7-(2,4-DIAMINO-6-ETHYLPYRIMIDIN-5-YL)-1-(3-METHOXYPROPYL)QUINOLINIUM 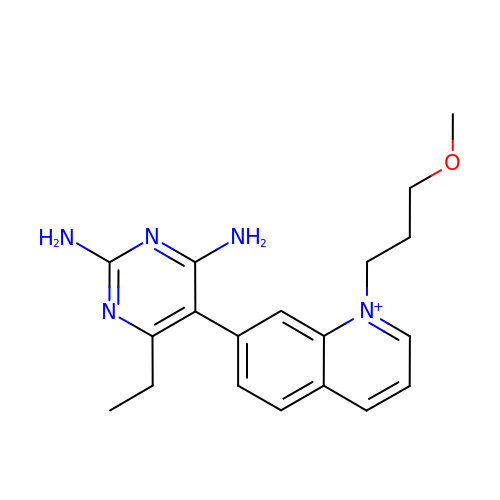| C19 H24 N5 O | AKHGQFJJDOXYFM-UHFFFAOYSA-O> MPKTPHTKGPDETLSLLADPYRFISRQCQRLGANAFESRFLLKKTNCLKGAKAAEIFYDTTRFE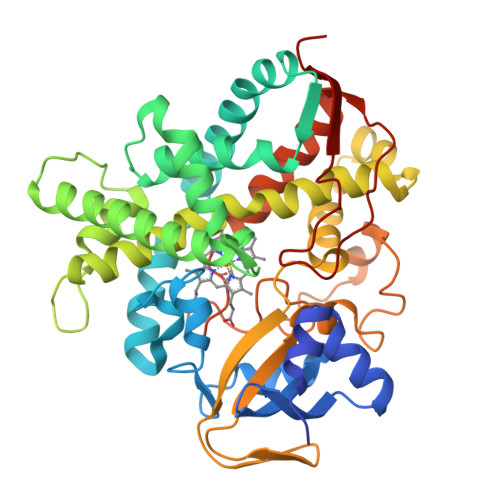REGAMPVAIQKTLLGQGGVQGLDGETHRHRKQMFMGLMTPERVRALAQLFEAEWRRAVPGWTRKGEIVFYDELHEPLTRAVCAWAGVPLPDDEAGNRAGELRALFDAAGSASPRHLWSRLARRRVDAWAKRIIEGIRAGSIGSGSGTAAYAIAWHRDRHDDLLSPHVAAVELVNVLRPTVHIAVYITFVAHALQTCSGIRAALVQQPDYAELFVQEVRRFYPFFPAVVARASQDFEWEGMAFPEGRQVVLDLYGSNHDAATWADPQEFRPERFRAWDEDSFNFIPQGGGDHYLGHRCPGEWIVLAIMKVAAHLLVNAMRYDVPDQDLSIDFARLPALPKSGFVMRNVHIGG The TREX-2 complex integrates mRNA nuclear export into the gene expression pathway and is based on a Sac3 scaffold to which Thp1, Sem1, Sus1, and Cdc31 bind. TREX-2 also binds the mRNA nuclear export factor, Mex67:Mtr2, through the Sac3 N-terminal region (Sac3N). Whereas protein transport is generally facilitated by karyopherin-β family proteins, mRNA export in yeast is mediated primarily by the Mex67:Mtr2 complex or in metazoans by NXF1:NXT1 (Segref et al., 1997; Braun et al., 2001). Mex67 is a modular protein containing four domains: RNA-recognition motif (RRM), leucine-rich repeat (LRR), nuclear transport factor 2-like (NTF2L), and ubiquitin-associated (UBA).

Diffraction quality crystals were obtained with ctSac31−20 and ctSac320−40. The complex with ctSac31−20 crystallized with P21 symmetry and the structure was determined to 1.8 Å resolution with Sac3 residues 15–20 (QVNNPF) clearly visible in the electron density, whereas the complex with ctSac320−40 crystallized with P212121 symmetry and the structure was determined to 1.85 Å with Sac3 residues 30–37 (SSVFGAPA) built into the model. Both crystal structures also contained the ctMex67 NTF2-like domain together with ctMtr2 and were refined to an Rfree of 19.3% and 20.3%, respectively, with excellent geometry. The Sac3N motifs bind primarily to the Mex67 NTF2L domain, and crystal structures of complexes between Mex67NTF2L:Mtr2 and Sac3N peptides identify a central role of the motif's Phe residue binding into a hydrophobic pocket on Mex67NTF2L. (2001) to which a PGFGQ peptide derived from nucleoporin NUP214 bound to NXF1, albeit with the chain direction reversed. This cavity was formed principally by Gly500, Leu501, Leu530, and Gly531, and accommodated a single Phe residue from either peptide (Phe20 and Phe33) with neighboring residues forming several direct and water-mediated hydrogen bonds. A conserved intrapeptide water-mediated H bond was seen in both Sac3N peptides, linking the Phe carbonyl to the carbonyls of Asn18 and Ser31, and the Sac3N20−40 peptide also contained a water-mediated H bond between the carbonyls of Gly34 and Ser31. Additional contacts were formed between Sac3N20−40 and the NTF2L domain, as the Phe residue bound was not at the C terminus of the peptide, with putative main-chain H bonds between Glu379Mex67 and Ala35Sac3, and a water-mediated H bond linking Asp377Mex67 and Ala37Sac3. Although the overall fold of the ctMex67 NTF2L domain or ctMtr2 was not altered by the binding of either ctSac3 peptide, a translation of the loop region of ∼3.0 Å prior to helix α1 of the NTF2L domain (residues 376–382, the pre-α1 loop) was observed for both peptides. However, in the ctSac3 peptides in the present study, a greater contribution was made by residues neighboring the bound Phe; as a result, this residue only contributed to 39% (ctSac31−20) and 35% (ctSac320−40) of the buried surface area.

> SPTPLPQLPSNVRDGENNVASTFLQAFFQLWDHDRLTLIPQFYDSETTFSVVFATDSPQDPASSSCSKFSRNLNILSPRHPSTLQRLFVGSNLIADLWKVLPATRHPSLDQTSQWLIDCHTFPHLADPTGMAPYAMGLMINVNGQCEEADISQNLYGTRTFSRCFILGPSKPGAPHPYRVLSDQLTLHTWKPQ;> MLSRRYAAKSFVEWYYRQINENKPVASGYVNNNATYTKAGHPPADITINGRVVATPEEWDTMLKEQRAQHNTSSSSTLPIGRKPVRYDVDCFDVHVINADYRFAAPQRMIEQHAPTDGVRMMMALTVSGSVYFGASPRSTDDYVIKQHFNDVFILVPNWDVLEKPGARSGRKYLIASHKYRAY;> FASPAPSNQGSSVFGAPAQST Trypanosoma brucei is the protozoan parasite that is the causative agent of Human African Trypanosomiasis (HAT), also known as African sleeping sickness. However, in T. brucei there are no enzymes for de novo synthesis and this parasite relies solely on its salvage pathways to make its purine nucleoside monophosphates. HGPRT is central to this salvage pathway, as it is responsible for the synthesis of IMP and GMP from hypoxanthine and guanine, respectively. Thus, the crystallographic and SEC-MALLS data agree in demonstrating that TbrHGPRT is dimeric.

In the crystal structures with GMP and 3 a dimer is observed in the asymmetric unit. In the TbrHGPRT.3 complex, 3 adopts two conformations resulting in the phosphonate group occupying alternative positions in the 5′-phosphate binding site. In one of these, the oxygen atoms of the phosphonate moiety form hydrogen bonds with the amide nitrogen atoms of D117 and L120, the amide nitrogen and side chain hydroxyl of T118 and the side chain hydroxyl of T121. In the second conformation, the phosphonate moiety is translated by ~1.8 Å, resulting in the formation of additional hydrogen bonds to the side-chain of E113 and the amide nitrogen of T121, and the removal of hydrogen bonds to the side chain hydroxyl and the amide nitrogen of T118. Three ordered water molecules are also found in or near this pocket. One forms a hydrogen bond with the amide nitrogen of T121 and a second forms a hydrogen bond with the side-chain of D117, thus making indirect links between the enzyme and the inhibitor, while the third water molecule makes networks with the surrounding ordered water molecules. As with GMP, the guanine base of 3 makes a π-π stacking interaction with the aromatic ring of F166, and forms hydrogen bonds to K145, the carbonyl oxygen of V167 and to the backbone carbonyl of D173. A sulphate ion is also present in this structure where the oxygen atoms form interactions with K54 and G55. In this structure, the bond between L53 and K54 is in the trans conformation and the side-chain of L53 is in hydrophobic contact with the carbon atoms of the linker in this ANP. The starting models for the complexes with GMP, IMP, 5 and 6 were based upon the refined model of the complex with 3.

>HHHHHHMEPACKYDFATSVLFTEAELHTRMRGVAQRIADDYSNCNLKPLENPLVIVSVLKGSFVFTADMVRILGDFGVPTRVEFLRASSYGHDTKSCGRVDVKADGLCDIRGKHVLVLEDILDTALTLREVVDSLKKSEPASIKTLVAIDKPGGRKIPFTAEYVVADVPNVFVVGYGLDYDQSYREVRDVVILKPSVYETWGKELERRKAAGEAKR[2x]> MARGLQGVMLRSFGARDHTATVIETISIAPHFVRVRMVSPTLFQDAEAEPAAWLRFWFPDPNGSNTEFQRAYTISEADPAAGRFAVDVVLHDPAGPASSWARTVKPGATIAVMSLMGSSRFDVPEEQPAGYLLIGDSASIPGMNGIIETVPNDVPIEMYLEQHDDNDTLIPLAKHPRLRVRWVMRRDEKSLAEAIENRDWSDWYAWATPEAAALKCVRVRLRDEFGFPKSEIHAQAYWNAGRAMGTHRATEPAATEPEVGAAPQPESAVPAPARGSWRAQAASRLLAPLKLPLVLSGVLAALVTLAQLAPFVLLVELSRLLVSGAGAHRLFTVGFAAVGLLGTGALLAAALTLWLHVIDARFARALRLRLLSKLSRLPLGWFTSRGSGSIKKLVTDDTLALHYLVTHAVPDAVAAVVAPVGVLVYLFVVDWRVALVLFGPVLVYLTITSSLTIQSGPRIVQAQRWAEKMNGEAGSYLEGQPVIRVFGAASSSFRRRLDEYIGFLVAWQRPLAGKKTLMDLATRPATFLWLIAATGTLLVATHRMDPVNLLPFMFLGTTFGARLLGIAYGLGGLRTGLLAARHLQVTLDETELAVREHPREPLDGEAPATVVFDHVTFGYRPGVPVIQDVSLTLRPGTVTALVGPSGSGKSTLATLLARFHDVERGAIRVGGQDIRSLAADELYTRVGFVLQEAQLVHGTAAENIALAVPDAPAEQVQVAAREAQIHDRVLRLPDGYDTVLGANSGLSGGERQRLTIARAILGDTPVLILDQATAFADPESEYLVQQALNRLTRDRTVLVIAHRLHTITRADQIVVLDHGRIVERGTHEELLAAGGRYCRLWDTGQGSRVAVAAAQDGTR;> MIRTWIALVPNDHRARLIGFALLAFCSVVARAVGTVLLVPLMAALFGEAPQRAWLWLGWLSAATVAGWVLDAVTARIGIELGFAVLNHTQHDVADRLPVVRLDWFTAENTATARQAIAATGPELVGLVVNLVTPLTSAILLPAVIALALLPISWQLGVAALAGVPLLLGALWASAAFARRADTAADKANTALTERIIEFARTQQALRAARRVEPARSLVGNALASQHTATMRLLGMQIPGQLLFSIASQLALIVLAGTTAALTITGTLTVPEAIALIVVMVRYLEPFTAVSELAPALESTRATLGRIGSVLTAPVMVAGSGTWRDGAVVPRIEFDDVAFGYDGGSG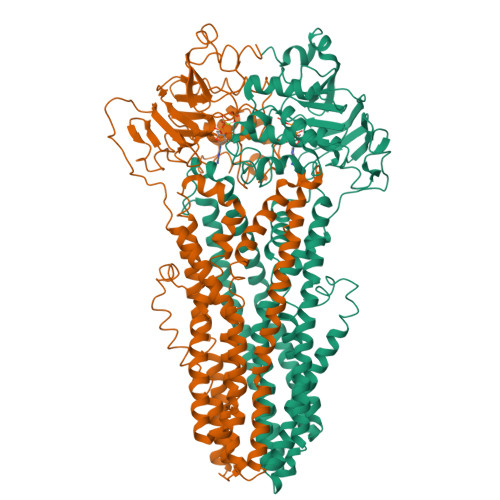PVLDGVSFCLQPGTTTAIVGPSGCGKSTILALIAGLHQPTRGRVLIDGTDVATLDARAQQAVCSVVFQHPYLFHGTIRDNVFAADPGASDDQFAQAVRLARVDELIARLPDGANTIVGEAGSALSGGERQRVSIARALLKAAPVLLVDQATSALDAENEAAVVDALAADPRSRTRVIVAHRLASIRHADRVLFVDDGRVVEDGSISELLTAGGRFSQFWRQQHEAAEWQILAE> SQLHYTVQEEQEHGTFVGNIAEDLGLDITKLSARGFQTVPNSRTPYLDLNLETGVLYVNEKIDREQ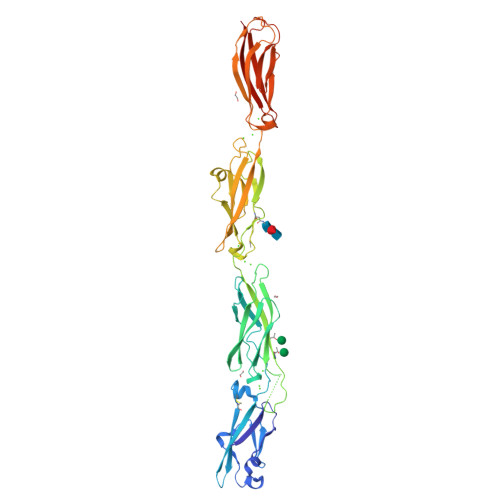ICKQSPSCVLHLEVFLENPLELFQVEIEVLDINDNPPSFPEPDLTVEISESATPGTRFPLESAFDPDVGTNSLRDYEITPNSYFSLDVQTQGDGNRFAELVLEKPLDREQQAVHRYVLTAVDGGGGGGVGEGGGGGGGAGLPPQQQRTGTALLTIRVLDSNDNVPAFDQPVYTVSLPENSPPGTLVIQLNATDPDEGQNGEVVYSFSSHISPRARELFGLSPRTGRLEVSGELDYEESPVYQVYVQAKDLGPNAVPAHCKVLVRVLDANDNAPEISFSTVKEAVSEGAAPGTVVALFSVTDRDSEENGQVQCELLGDVPFRLKSSFKNYYTIVTEAPLDREAGDSYTLTVVARDRGEPALSTSKSIQVQVSDHHHHHH[3-[[4-[6-chloranyl-2-(1,3-dimethylpyrazol-4-yl)-3H-imidazo[4,5-b]pyridin-7-yl]pyrazol-1-yl]methyl]phenyl]-(4-methylpiperazin-1-yl)methanone | C27 H28 Cl N9 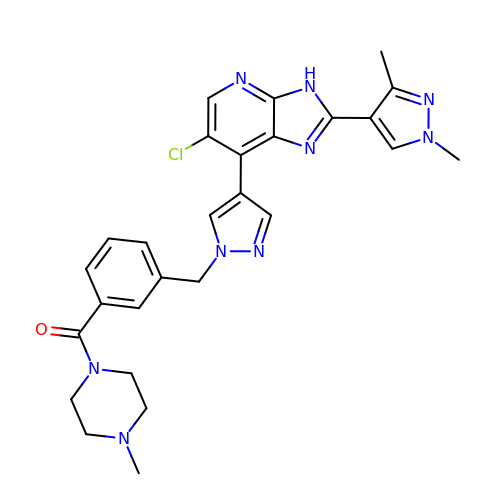O | MBQJFWXFLPQAID-UHFFFAOYSA-N> MQLNNRDLKSIIDNEALAYAMYTVENRAIPNMIDGFKPVQRFVIARALDLARGNKDKFHKLASIAGGVADLGYHHGENSAQDAGALMANTWNNNFPLLDGQGNFGSRTVQKAAASRYIFARVSKNFYNVYKDTEYAPVHQDKEHIPPAFYLPIIPTVLLNGVSGIATGYATYILPHSVSSVKKAVLQALQGKKVTKPKVEFPEFRG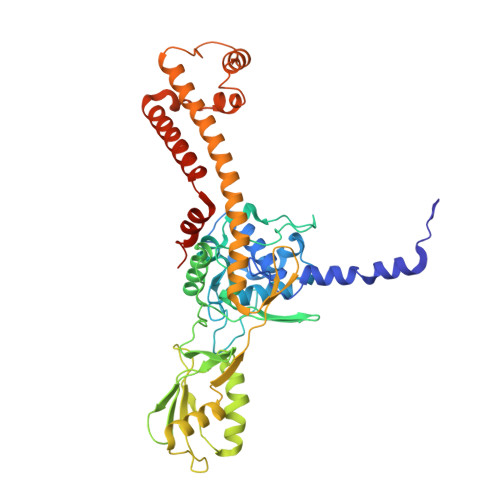EVVEIDGQYEIRGTYKFTSRTQMHITEIPYKYDRETYVSKILDPLENKGFITWDDACGEHGFGFKVKFRKEYSLSDNEEERHAKIMKDFGLIERRSQNITVINEKGKLQVYDNVVDLIKDFVEVRKTYVQKRIDNKIKETESAFRLAFAKAHFIKKVISGEIVVQGKTRKELTEELSKIDMYSSYVDKLVGMNIFHMTSDEAKKLAEEAKAKKEENEYWKTTDVVTEYTKDLEEIKHHHHHHHHHH> MALLAEHLLKPLPADKQIETGPFLEAVSHLPPFFDCLGSPVFTPIKDVISGNITKIKAVYDTNPAKFRTLQNILEVEKEMYGAEWPKVGATLALMWLKRGLRFIQVFLQSICDGERDENHPNLIRVNATKAYEMALKKYHGWIVQKIFQAALYAAPYKSDFLKALSKGQNVTEEECLEKIRLFLVNYTATIDVIYEMYTQMNAELNYKV

Human glycolipid transfer protein (hsGLTP) forms the prototypical GLTP fold and is characterized by a broad transfer selectivity for glycosphingolipids (GSLs). In human GLTP, a glycolipid headgroup recognition centre located on the protein surface enables selective binding of the GSL head and ceramide amide groups via multiple specific interactions. Encapsulation of lipid chains within the hydrophobic pocket involves a cleft-like gating mechanism that results in two glycolipid-binding modes. To elucidate the structural dynamics of the GLTP–GSL dimer and associated adaptations, we comparatively analyzed nine novel crystal structures of wild-type GLTP (wtGLTP) and the sulfatide-specific mutants D48V and A47D/D48V complexed with N-lauroyl-containing monosulfatide (N-lauroyl-3-O-sulfo-galactosylceramide; hereafter referred to as 12:0 monoSF) and disulfatide (N-lauroyl-3,6-di-O-sulfo-galactosylceramide; hereafter referred to as 12:0 diSF) in different crystal forms and compared them with previously studied GLTP–24:1 monoSF complexes.

Because the double mutation A47D/D48V restores the open dimer conformation along with the local negative charge repulsion in the dimer, we also studied the crystal structure of the double mutant A47D/D48V complexed with 12:0 monoSF. The mutations D48V and A47D/D48V, which reversibly regulate access of sphingosine to the hydrophobic pocket, mediate the regulation in the disulfatide (12:0 diSF) differently compared with the monosulfatide (12:0 monoSF) or in the short-acyl-chain sulfatide (12:0 monoSF) compared with the long-acyl-chain sulfatide (24:1 monoSF). Similarly, SF complexes with mutant D48V systematically deviate from those with wtGLTP or the double mutant A47D/D48V.5-[(2E,4aR,7aR)-6-(4-ethoxy-5-fluoro-6-methylpyrimidin-2-yl)-2-imino-3-methyl-4-oxooctahydro-7aH-pyrrolo[3,4-d]pyrimidin-7a-yl]thiophene-2-carbonitrile 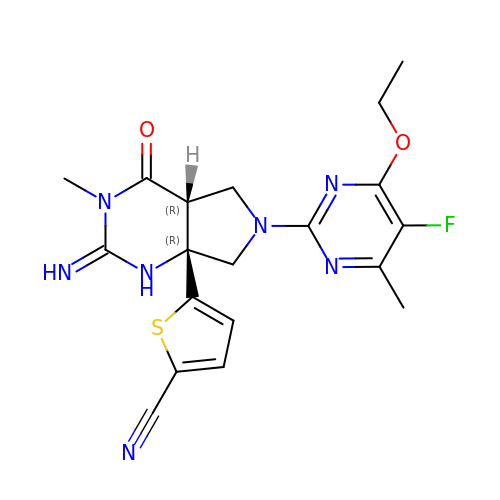| C19 H20 F N7 O2 S | NAIWJSDALLQSJO-BUXKBTBVSA-N> HHHHHHSSGHKEKLHTLEEFSYEFFRAPEKDAVSMAVLPLARARGHLWAYSCEPLRQPLLKRVHANVDLWDIACQIFVAILRYMGDYPSRQAWPTLELTDQIFTLALQHPALQDEVYCQILKQLTHNSNRHSEERGWQLLWLCTGLFPPSKGLLPHAQKFIDTRRGKLLAPDCSRRIQKVLRTGPRKQPPHQVEVEAAEQNVSRICHKIYFPND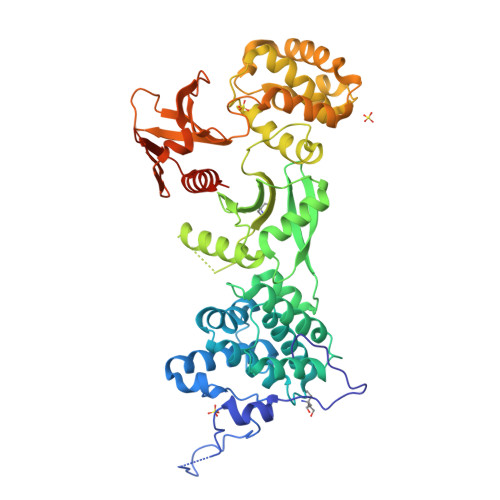TSEMLEVVANTRVRDVCDSIATRLQLASWEGCSLFIKISDKVISQKEGDFFFDSLREVSDWVKKNKPQKEGAPVTLPYQVYFMRKLWLNISPGKDVNADTILHYHQELPKYLRGFHKCSREDAIHLAGLIYKAQFNNDRSQLASVPKILRELVPENLTRLMSSEEWKKSILLAYDKHKDKTVEEAKVAFLKWICRWPTFGSAFFEVKQTSEPSYPDVILIAINRHGVLLIHPKTKDLLTTYPFTKISSWSSGSTYFHMALGSLGRGSRLLCETSLGYKMDDLLTSYVQQLLSAMNKQRGSKAPALAST> EAEPGAAEFAALRNRWVDQITGRNVIQAGDPDFAKAITALNNKAADSLAKLDVKKGRTSVFTDLSLAKDAEMVTTYTRLSQLATAWATPTAAVFGDAAVLAAIKAGLADANTLCYNDRKEEVGNWWSWEIGVPRALADAMVLLHAELSAAERTAYCAAIDHFVPDPWLQFPPKRGKITSVGANRVDLCQGIIIRSLAGEDPTKLNHAVAGLSQVWQYVTSGDGIFRDGSFIQHSTTPYTGSYGVVLLTGLSKLFSLLGGTAFEVSDPTRSIFFDAVEGSFAPVMINGAMADAVRGRSISREANTGYDLGASAIEAILLLARAMDPATAARWRGLCAGWIARDTYRPILNSASVPRTALVKQLEATGVAPVAEATGHKLFPAMDRTMHRGPGWALSLALSSNRIAWYECGNGENNRGYHTGSGMTYFYTSDLGQYDDAFWATANYNRLPGITVDTTPLPDKVEGQWGAAVPADEWSG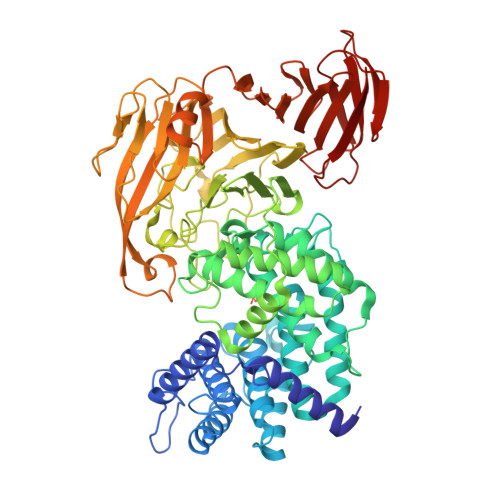ATALGEVAAVGQHLVGPGRTGLTARKSWFVSGDVTVCLGADISTASGAKVETIVDHRNLHQGSNTLTTAAGTIAGTAGTVEVLGDGRWVHLEGFGGYAMLDDSPLHVLRETRSGSWSGVNINGSATVQQRNFATLYVNHGVGPVAGSYAYMVAPGASVDLTRKLLEGNKYSVIRNDATAQSVEFKTAKTTAATFWKPGMAGDLGASGPACVVFSRHGNELSLAVSEPTQKAAGLTLTLPEGTWSSVLEGAGTLGTDADGRSTLTLDTTGLSGKTKLIKLKR> MSNTTWGLQRDITPRLGARLVQEGNQLHYLADRASITGKFSDAECPKLDVVFPHFISQIESMLTTGELNPRHAQCVTLYHNGFTCEADTLGSCGY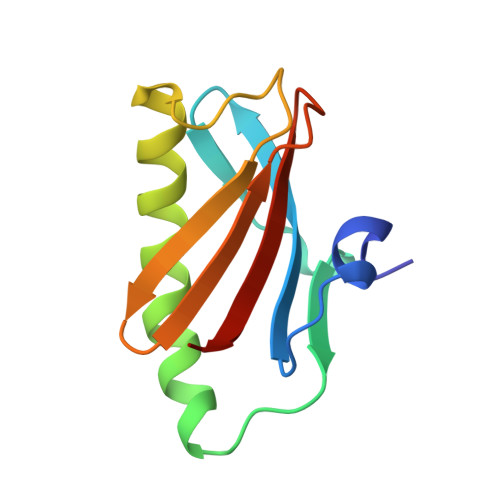VYIAVYPTQR> GDELYRQSLEIISRYLREQATGAKDTKPMGRSGATSRKALETLRRVGDGVQRNHETAFQGMLRKLDIKNEDDVKSLSRVMIHVFSDGVTNWGRIVTLISFGAFVAKHLK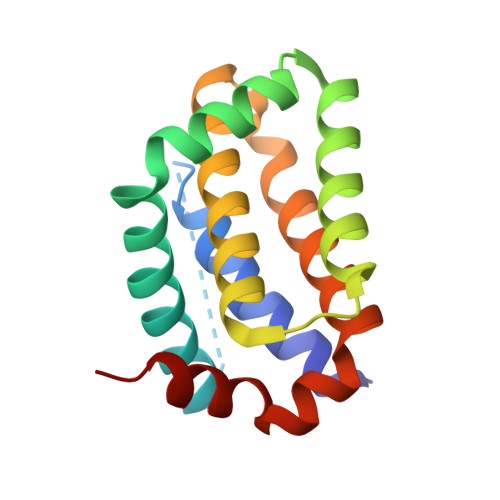TINQESCIEPLAESITDVLVRTKRDWLVKQRGWDGFVEFFHV> SAVKLSYDEAYDNPSSSLLSVTCSDGENGLYPKYRTFGDLPGFPCIGGSSDIAGYNSPNCGSCYQLTYSSAHTTPKSIYMVAIDRSAEGFTASKQAMDDLTNKRAEE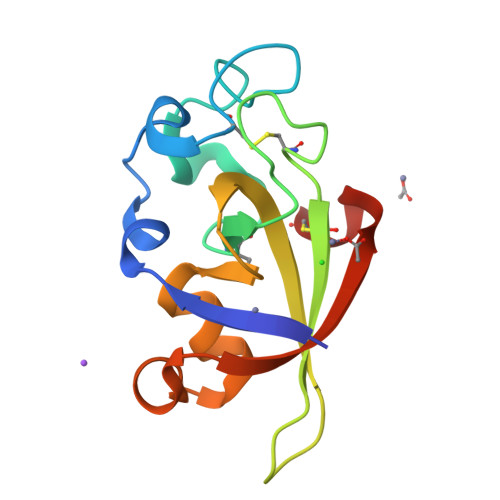LGTVNVDVRKVDFSRCERKS>[3x]MGAMIVKEVYETAEKIKSMEIRGAGRIARAAAQALMIQAEKSKAKEPEELWNELKVASKILYNTRPTAVSLPNALRYVMHRVKAAYLGGADLETLRFTAINSAKEFIYNSEKAIERIGEIGAKRIEDGDIIMTHCHSKAAISVMKKAFEQGKNIKVIVTETRPKWQGKITAKELASYGIPVIYIVDSAARHYMKMTDKVVMGADSITANGAVINKIGTSLIALTAKEHRVWVMIAAETYKFHPATMLGQLVEIEMRDPTEVIPEEELRTWPKNIEVWNPAFDVTPPEYIDVIITERGIIPPYAAIDILKEEFGWALKYKEPWED

In summary, our study demonstrates that PH0208 protein would function as a purine nucleotide dependent R15Pi enzyme and not as a homologue of the regulatory subunit of eIF2B. In NMP degradation pathway, R15Pi catalyzes the conversion of ribose-1,5-bisphosphate (R15P, substrate) into ribulose-1,5-bisphosphate (RuBP, product) in an adenosine 5′-monophosphate (AMP)-dependent manner. AMP acts as an activator of R15Pi and in its absence the enzymatic activity has been found to decline dramatically. Monomer of PH0208 protein consists of an N-terminal α-helical domain (residues 1–122) and a C-terminal α-β-α sandwich domain (residues 123–324).

Thus, we determined the structure of PH0208 protein in complex with AMP molecule. The binding site of AMP lies at the interface of three monomers (chain A, B and D) of the hexameric protein. The side chains of Arg124 and Asp290 of chain A undergoes a shift towards AMP to form hydrogen bond with the O2′ and O3′ oxygen atoms of the ribose sugar. Another two residues of chain A, Arg229 and Trp231 are involved in interacting with the phosphate groups of the AMP molecule. The side chain atoms of Asn209 and the backbone atoms of Val251 of chain B forms hydrogen bond with the oxygen (O2′ and O3′) atoms of the ribose sugar and the nitrogen (N1 and N6) atom of the adenosine base ring, respectively. Along with chain A and chain B, AMP also binds to a third protomer of the hexameric protein through interactions involving the side chain atoms of Arg190 and Lys194 of chain D. Thus, one AMP molecule positions itself to hold three protomers of the hexamer. All the amino acid residues of PH0208 protein forming hydrogen bond with AMP are found to be absolutely conserved in R15Pi enzymes. The positioning of the AMP at the interface of three monomers implies that AMP might play an important role in providing conformational stability to the hexameric form of PH0208 protein. The change in the side chain orientation of Arg124 and Asp290 to interact with AMP portrays as the key interactions required for this stabilization.>[2x]TVESNWG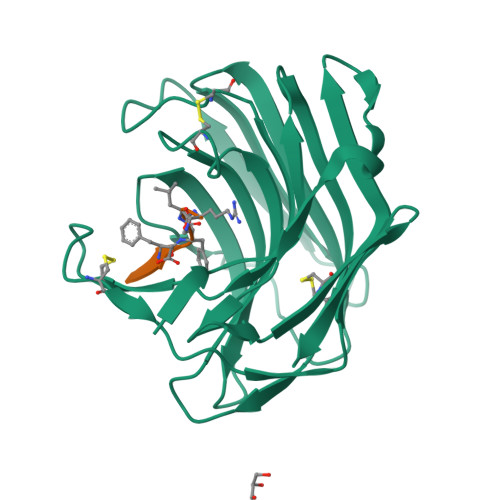GAILIGSDFDTVSATANVPSASGGSSAAGTAWVGIDGDTCQTAILQTGFDWYGDGTYDAWYEWYPEVSDDFSGITISEGDSIQMSVTATSDTSGSATLENLTTGQKVSKSFSNESSGSLCRTNAEFIIEDFEECNSNGSDCEFVPFASFSPAVEFTDCSVTSDGESVSLDDAQITQVIINNQDVTDCSVSGTTVSCSYV;>[2x]XFKFFLR HHV-6B U14 is a tegument protein essential for viral propagation, and additionally it interacts with host factors such as tumor suppressor p53 and cellular protein EDD, thereby regulating host cell responses. HHV-6B U14 is a tegument protein that is 604 amino acid residues in length. U14 belongs to the herpes pp85 superfamily that is shared among beta herpesviruses, and has no homologs in alpha and gamma herpesvirus. The N-terminal domain of U14 (U14-NTD) adopts an elongated, helix-rich fold without any significant overall similarity to known structures.

The structures of native U14-NTD and the SeMet-derivative were determined at 1.85 Å and 2.3 å resolutions, respectively. There were two almost identical U14-NTD molecules in the asymmetric unit. Almost all of the U14-NTD residues were assigned to the electron density, with the exception of N-terminal residues 1–7 and C-terminal residues 456–458, indicating that the designed U14-NTD represents an actual structural domain of U14. U14-NTD has an elongated helix-rich structure composed of sixteen α helices, four 310 helices and two β strands. To facilitate structure description, the U14-NTD structure was divided into four subdomains (SDs) based on secondary structure topology and spatial arrangement. In the crystal structure, a dimer is formed along the long axis of U14-NTD in an antiparallel orientation. The calculated buried surface area per monomer is 4146 Å2 (red), which is a relatively large value compared with those of known homodimer structures of similar size, at approximately 2800 Å2. One noticeable characteristic of the U14-NTD dimer is an internal cavity within the dimer interface. Broadly spanning electrostatic interactions contribute to the dimerization. The HHV-6B U14 structure suggests multiple structural features as potential function sites, such as the negatively- and positively-charged clusters, the β hairpin flanked by the hydrophobic patch, and the grooves formed along the dimer interface.

>GPEGSKTFNIPTFVLDENCNFIPDVLSRANAKFIKEVLIRDSYNAVCLANSFIPMATQTVEQILIIITKFKFSRSRDLLMSVFRLGVHINRFYAGKNQVKHMITMMKSLFDTEEAMRQLDRALMGLFVDARDNSYMPLIALSLHENGLPDSKFIKAVRLIQTTVNSFHNRPDADIEQYAEKLRAYNYLYKIPKYTLKEAVDIYSDNLKDLTIGVNKKPTLLFTSSDDAYLSHIYNDLLFLTSTWNMIYNCKKEIRRLNTWIKYEINSIMETAVLVGFQLPDLKETILDLAALISNMNLVSPDKELFPHYKLILAKLFEICIFATKANICILPSFIKGHLIEFEDVLKRSNDDEDLNYLLLKSRDSDDEYDEDKPPIQVDPGRVDNVLTDSDFFNVTPENAFSSIAIMPISYDKTIDVEDNEIQVLEVEMQSLSAVVYGAVASKYGLSLEQVIRKLNQNE[2x]uridine uronic acid | C9 H10 N2 O7 | 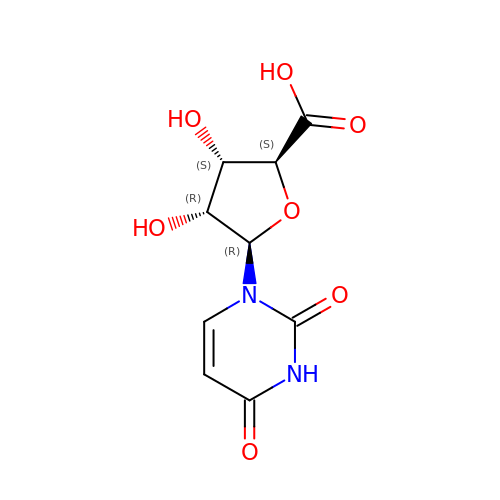BMDRRZMODBSOPT-BNHYGAARSA-N>MSLQLVKKFQKRLEDIVAYGGTRNESSVRAAFQQLLSDWAEGSGLRLITEVTQKAVAGNNVRPDGTLKDSLQQSRGYWESKDEADTLDDEIQKKLAKGYPRDNIIFEDSRLAVLMQNGEEVQRVDMGDAGALAGLLKLFFEFEPPQVLEFRKAVDHFKDEMPHLLKILREAADAAEQKADYRGERDHFVEIAKEAINPDFSPRDAREMLIQHILTGDLFTSVFDNAQYHEDNNIAQQLQQLAATFYKGPVKRDIAERTKRYYGAIQAAAAQIADHHEKQRFLKALYENFYRAYNPAGAERLGIFYTPGEIVRFMIEATDTLLEKHFQKELADKGVEILDPATGTGTFITELIDFLPKAKLEQKYREELHCNELALLPYYIANLNIEATYAQKMGRYEEFRNIVLVDTLDNTGFGVHGQQSGLFGSVTAENLERAKRQNARPVRVIIGNPPYRANQANENDNNKNREYKEIDRRIKATYVAASTAQKTKLYDMYSR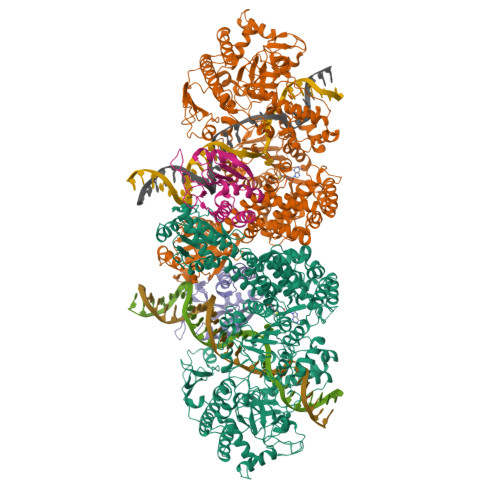FLRWATDRLKEDGIVAFVSNSSFIDSRTFDGFRKEVVKDFDHIYILDMKGNANTSGERRKREGGNVFNDQIKVGVAVYFLVRSAAGKRKSKDTKIWYHAVPDFWRAREKLEWLKTTKFEDIEFDHIRPDAKHNWLGQVDEENDWNEFLPVADKDTKQAKGLGQERAIFKLYSLGVVTNRDEWVYSRAEDELADKVRYFIGRYNEIIKLPLGDLMSRNWEGDIKMTRATIADAQSRKSYSLEKNSIVPSLYRPFDVLKMYFSKNLNEMQYQMPSIFPKGVGENVVIALSGSPAAKPFQVLATDILPSLDLLEKTQCLPFYRYTMNGERLNNITDYALKAFQTHYADTSISREDIFHYVYAVLHHPAYREKYALNLRQEFPRIPFYPEFGRWAAWGRELMALHIGFESVAPYPLKRTDEPPKNDTPEALALAKKARLKVQRDAAKQPTGAVELDGLTTLAGIPAAAWAYKLGNRSALEWVLERHKETTPKDATIREKFNTYRFADHKERVIDLLARVTTVSVETVRIVGEMPAETM[4x]2-(4'-CARBAMIMIDOYL-2'-HYDROXYBIPHENYL-4-YL)-1H-BENZIMIDAZOLE-5-CARBOXIMIDAMIDE | C21 H18 N6 O | 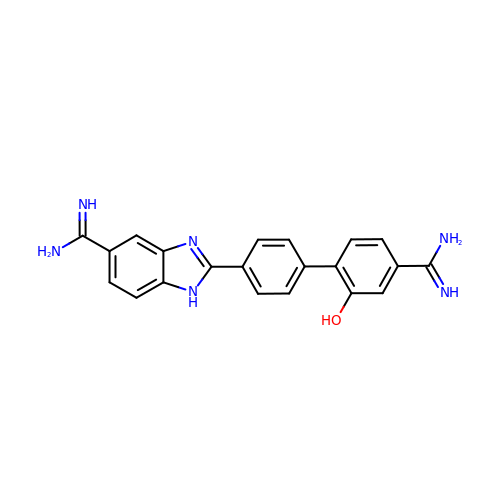VYJOWVQQJBILOA-UHFFFAOYSA-N(azepan-1-yl)(2-{[(furan-2-yl)methyl]amino}-6-methylpyridin-3-yl)methanone | C18 H23 N3 O2 | 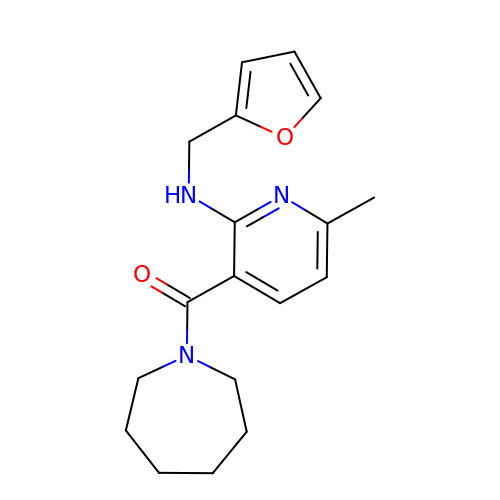JCTPWJNVLSRFOU-UHFFFAOYSA-N> MMVISEKVRKALNDQLNREIYSSYLYLSMATYFDAEGFKGFAHWMKKQAQEELTHAMKFYEYIYERGGRVELEAIEKPPSNWNGIKDAFEAAL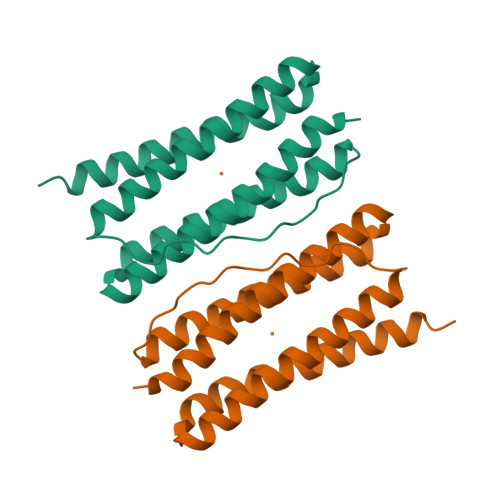KHEEFVTQSIYNILELAHEEKDHATVSFLKWFVDEQVEEEDQVREILDLLEKANG>[4x]SNANEWQEKPSWNTHFSEHKAQGVIVLWNENKQQGFTNNLKRANQAFLP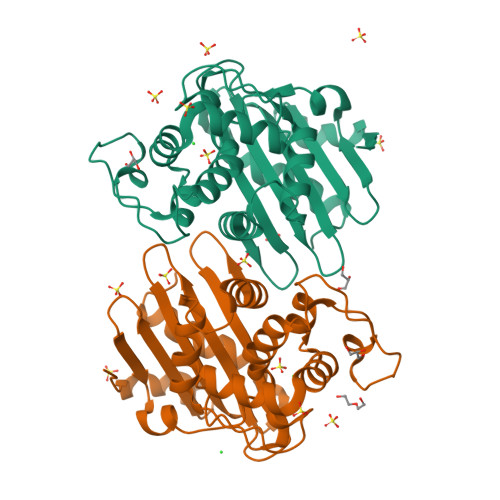ASTFKIPNSLIALDLGVVKDEHQVFKWDGQTRDIAAWNRDHDLITAMKYSVVPVYQEFARQIGQARMSKMLHAFDYGNEDISGNLDSFWLDGGIRISATEQVAFLRKLYHNKLHVSERSQRIVKQAMLTEANSDYIIRAKTGYSTRIEPQIGWWVGWVELDDNVWFFAMNMDMPTADGLGLRQAITKEVLKQEKIIP1-[(6,8-dimethyl-2-oxo-1,2-dihydroquinolin-3-yl)methyl]-1-(2-hydroxyethyl)-3-(4-hydroxyphenyl)thiourea | C21 H23 N3 O3 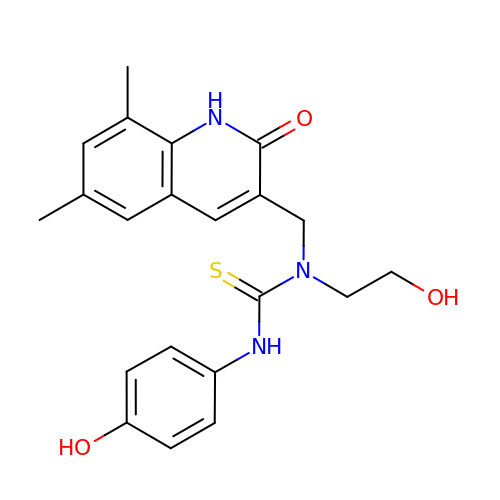S | GJJDKMIHKNXATK-UHFFFAOYSA-N>[4x]MGSSHHHHHSSGENLYFQGHMKHGIYYSYWEHEWSAKFGPYIEKVAKLGFDIIEVAAHHINEYSDAELATIRKSAKDNGIILTAGIGPSKTKNLSSEDAAVRAAGKAFFERTLSNVAKLDIHTIGGALHSYWPIDYSQPVDKAGDYARGVEGINGIADFANDLGINLCIEVLNRFENHVLNTAAEGVAFVKDVGKNNVKVMLDTFHMNIEEDSFGDAIRTAGPLLGHFHTGESNRRVPGKGRMP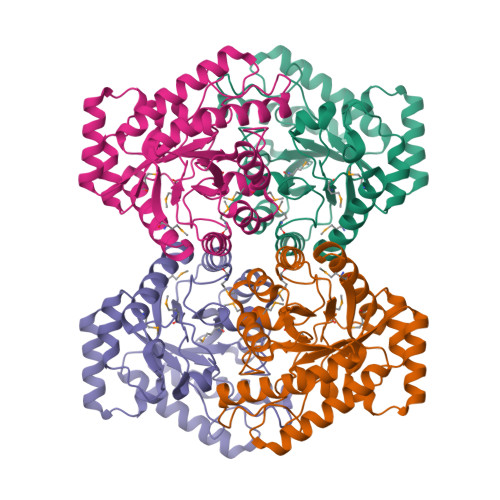WHEIGLALRDINYTGAVIMEPFVKTGGTIGSDIKVWRDLSGGADIAKMDEDARNALAFSRFVLGG>MGCWGRNRGRLLCMLALTFMFMVLEVVVSRVTSSLAMLSDSFHMLSDVLALVVALVAERFARRTHATQKNTFGWIRAEVMGALVNAIFLTGLCFAILLEAIERFIEPHEMQQPLVVLGVGVAGLLVNVLGLCLFHHHSGFSQDSGHGHSHGGHGHGHGLPKGPRVKSTRPGSSDINVAPGEQGPDQEETNTLVANTSNSNGLKLDPADPENPRSGDTVEVQVNGNLVREPDHMELEEDRAGQLNMRGVFLHVLGDALGSVIVVVNALVFYFSWKGCSEGDFCVNPCFPDPCKAFVEIINSTHASVYEAGPCWVLYLDPTLCVVMVCILLYTTYPLLKESALILLQTVPKQIDIRNLIKELRNVEGVEEVHELHVWQLAGSRIIATAHIKCEDPTSYMEVAKTIKDVFHNHGIHATTIQPEFASVGSKSSVVPCELACRTQCALKQCCGTLPQAPSGKDAEKTPAVSISCLELSNNLEKKPRRTKAENIPAVVIEIKNMPNKQPESSL[2x]

Among the ten hZnT members, hZnT1 is the only Zn2+ transporter predominantly located on the plasma membrane, mediating Zn2+ efflux from the cytosol to extracellular environments, to protect cells against Zn2+ toxicity. The overall structure of hZnT1 adopts a “mushroom”-shaped homodimeric architecture with the transmembrane domain (TMD) and cytosolic domain (CTD) of two protomers tightly packed. Each hZnT1 protomer comprises three parts: an extracellular domain (ECD), a TMD and a cytosolic CTD. The second part TMD of each hZnT1 protomer contains six transmembrane helices (TM1–6), forming a Zn2+ transport pathway.

The first region ECD (residues 271–312) is formed by the linker between TM5 and TM6, mediates intersubunit dimerization through hydrophobic interactions, a feature not observed in other ZnT family members. The distinctive extracellular cysteine-rich ECD in hZnT1 formed an inter-subunit disulfide bond (C291–C291) and two intra-subunit disulfide bonds (C276–C282, C286–C311). This unique arrangement is primarily responsible for sequestering extracellular Cu2+ and facilitating their efficient transport, while exhibiting minimal impact on Zn2+ transport, which expands the extra physiological function of hZnT1 beyond its role as Zn2+/H+ and Zn2+/Ca2+ exchanger. Specially, residues of TM2 and TM3 interdigitate at the dimer interface and establish a complex network of hydrophobic interactions to promote the dimer formation in the TMD. The transmembrane helices TM2, TM3, TM5 and TM6 are tightly bundled at the cytosolic half of the TMD in both protomers, and collectively create a cavity that is solvent accessible from the extracellular milieu but entirely sealed from the cytoplasmic side, indicating that our hZnT1 structure is in an OF state. Additionally, a His-rich loop flanked by TM4 and TM5 is located on the cytosolic side, with the majority invisible due to its flexible nature, except residues 134–136 near the C-terminal end of TM4 and residues 228–232 near the N-terminal end of TM5 build according to the map density. The last region CTD (residues 345–507) is composed of two short α helices (α1–2) and three paralleled β sheets (β1–3), contributing the extensive interactions to stabilize the dimeric state of hZnT1. Exquisitely, the β sheets of one protomer tightly pack against that of another protomer through hydrophobic interactions and four hydrogen bonds between H387–T415 and I417–Q418. In addition, K69, N70, and T71 in the extended loop between TM2–TM3 protrude into the neighboring subunit and tuck into the pocket between β1 and the loop of TM6-α1, establishing pivotal hydrogen bonds with L344, V347, and V374 to further strengthen the stability of hZnT1 homodimer. Superimposing the apo and CDDO-ME bound hZnT1 structures illustrated a noticeable significant movement of H43 and E99, which also substantiates that these conformational changes are indeed attributable to the binding of the inhibitor.> GGRGGRGRHPGHLKGREIGLWYAKKQGQKNKEAERQERAVVHMDERREEQIVQLLHSVQTKNDKDEEAQISWFAPEDHGYGTEAPAENKPNSVKNVEHQAAAMINQEKRPFRIRDKYIDRDSEYLLQENEPDATLDQQLLEDLQKKKTDLRYIEMQRFREKLPSYGMQKELVNMIDNHQVTVISGETGCGKTTQVTQFILDNYIERGKGSACRIVCTQPRRISAISVAERVAAERAESCGNGNSTGYQIRLQSRLPRKQGSILYCTTGIILQWLQSDPHLSSVSHIVLDEIHERNLQSDVLMTVVKDLLSYRPDLKVVLMSATLNAEKFSEYFGNCPMIHIPGFTFPVVEYLLEDIIEKIRYVPEQKEHRSQFKKGFMQGHVNRQEKEEKEAIYKERWPGYLRELRQRYSASTVDVVEMMDDEKVDLNLIAALIRYIVLEEEDGAILVFLPGWDNISTLHDLLMSQVMFKSDKFIIIPLHSLMPTVNQTQVFKRTPPGVRKIVIATNIAETSITIDDVVYVIDGGKIKETHFDTQNNISTMSAEWVSKANAKQRKGRAGRVQPGHCYHLYNSLRASLLDDYQLPEILRTPLEELCLQIKILRLGGIAHFLSRLMDPPSNEAVLLSIKHLMELNALDKQEELTPLGVHLARLPVEPHIGKMILFGALFCCLDPVLTIAASLSFKDPFVIPLGKEKVADARRKELAKDTKSDHLTVVNAFKGWEKAKQRGFRYEKDYCWEYFLSSNTLQMLHNMKGQFAEHLLGAGFVSSRNPQDPESNINSDNEKIIKAVICAGLYPKVAKIRLNLGKKRKMVKVYTKTDGVVAIHPKSVNVEQTEFNYNWLIYHLKMRTSSIYLYDCTEVSPYCLLFFGGDISIQKDNDQETIAVDEWIIFQSPARIAHLVKELRKELDILLQEKIESPHPVDWKDTKSRD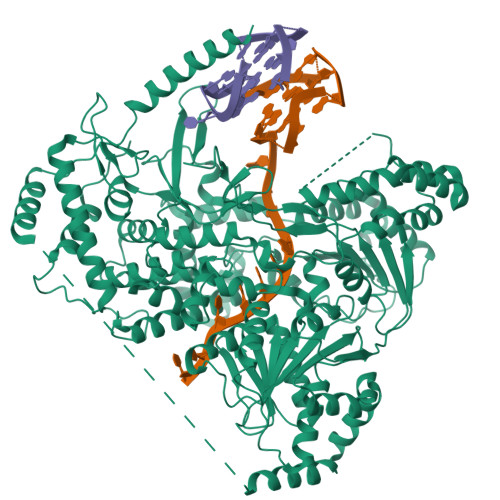CAVLSAIIDLIKTQEKATPRNLPPRFQDGYYSPHHHHHHHH>[3x]ANPLYQKHIISINDLSRDDLNLVLATAAKLKANPQPELLKHKVIASCFFEASTRTRLSFETSMHRLGASVVGFSDS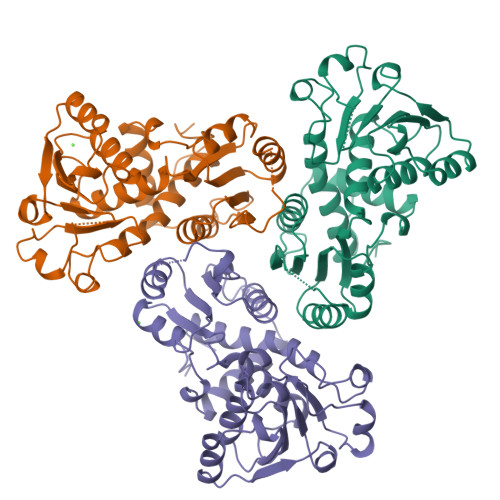ANTSLGKKGETLADTISVISTYVDAIVMRHPQEGAARLATEFSGNVPVLNAGDGSNQHPTQTLLDLFTIQETQGRLDNLHVAMVGDLKYGRTVHSLTQALAKFDGNRFYFIAPDALAMPQYILDMLDEKGIAWSLHSSIEEVMAEVDILYMTRVQKERLDPSEYANVKAQFVLRASDLHNAKANMKVLHPLPRVDEIATDVDKTPHAWYFQQAGNGIFARQALLALVLNRDLVL> MDYDFKVKLSSERERVEDLFEYEGCKVGRGTYGHVYKAKRKDGKDDKDYALKQIEGTGISMSACREIALLRELKHPNVISLQKVFLSHADRKVWLLFDYAEHDLWHIIKFHRASKANKKPVQLPRGMVKSLLYQILDGIHYLHANWVLHRDLKPANILVMGEGPERGRVKIADMGFARLFNSPLKPLADLDPVVVTFWYRAPELLLGARHYTKAIDIWAIGCIFAELLTSEPIFHCRQEDIKTSNPYHHDQLDRIFNVMGFPADKDWEDIKKMPEHSTLMKDFRRNTYTNCSLIKYMEKHKVKPDSKAFHLLQKLLTMDPIKRITSEQAMQDPYFLEDPLPTSDVFAGCQIPYPKREFLTEEEPDDKGDKKNQQQQQGNNHTNGTGHPGNQDSSHTQGPPLKKVRVVPPTTTSGGLIMTSDYQRSNPHAAYPNPGPSTSQPQSSMGYSATSQQPPQYSHQTHRY;> MAGNFWQSSHYLQWILDKQDLLKERQKDLKFLSEEEYWKLQIFFTNVIQALGEHLKLRQQVIATATVYFKRFYARYSLKSIDPVLMAPTCVFLASKVEEFGVVSNTRLIAAATSVLKTRFSYAFPKEFPYRMNHILECEFYLLELMDCCLIVYHPYRPLLQYVQDMGQEDMLLPLAWRIVNDTYRTDLCLLYPPFMIALACLHVACVVQQKDARQWFAELSVDMEKILEIIRVILKLYEQWKNFDERKEMATILSKMPKPKPPPNSEGEQGPNGSQNSSYSQS;> MAAFGILSYEHRPLKRPRLGPPDVYPQDPKQKEDELTALNVKQGFNNQPAVSGDEHGSAKNVSFNPAKISSNFSSIIAEKLRCNTLPDTGRRKPQVNQKDNFWLVTARSQSAINTWFTDLAGTKPLTQLAKKVPIFSKKEEVFGYLAKYTVPVMRAAWLIKMTCAYYAAISETKVKKRHVDPFMEWTQIITKYLWEQLQKMAEYYRPGPAGSGGCGSTIGPLPHDVEVAIRQWDYTEKLAMFMFQDGMLDRHEFLTWVLECFEKIRPGEDELLKLLLPLLLRYSGEFVQSAYLSRRLAYFCTRRLALQLDGVSSHSSHVISAQSTSTLPTTPAPQPPTSSTPSTPFSDLLMCPQHRPLVFGLSCILQTILLCCPSALVWHYSLTDSRIKTGSPLDHLPIAPSNLPMPEGNSAFTQQVRAKLREIEQQIKERGQAVEVRWSFDKCQEATAGFTIGRVLHTLEVLDSHSFERSDFSNSLDSLCNRIFGLGPSKDGHEISSDDDAVVSLLCEWAVSCKRSGRHRAMVVAKLLEKRQAEIEAERCGESEAADEKGSIASGSLSAPSAPIFQDVLLQFLDTQAPMLTDPRSESERVEFFNLVLLFCELI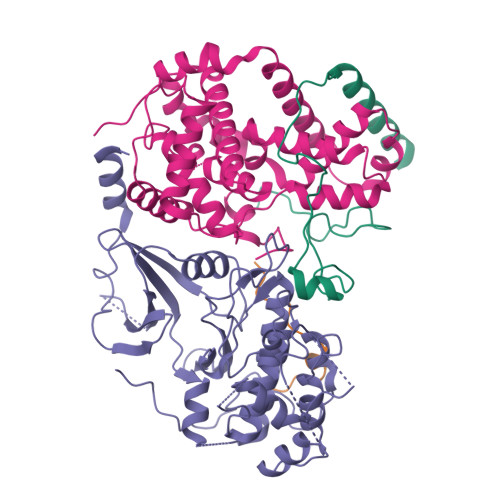RHDVFSHNMYTCTLISRGDLAFGAPGPRPPSPFDDPADDPEHKEAEGSSSSKLEDPGLSESMDIDPSSSVLFEDMEKPDFSLFSPTMPCEGKGSPSPEKPDVEKEVKPPPKEKIEGTLGVLYDQPRHVQYATHFPIPQEESCSHECNQRLVVLFGVGKQRDDARHAIKKITKDILKVLNRKGTAETDQLAPIVPLNPGDLTFLGGEDGQKRRRNRPEAFPTAEDIFAKFQHLSHYDQHQVTAQVSRNVLEQITSFALGMSYHLPLVQHVQFIFDLMEYSLSISGLIDFAIQLLNELSVVEAELLLKSSDLVGSYTTSLCLCIVAVLRHYHACLILNQDQMAQVFEGLCGVVKHGMNRSDGSSAERCILAYLYDLYTSCSHLKNKFGELFSDFCSKVKNTIYCNVEPSESNMRWAPEFMIDTLENPAAHTFTYTGLGKSLSENPANRYSFVCNALMHVCVGHHDPDRVNDIAILCAELTGYCKSLSAEWLGVLKALCCSSNNGTCGFNDLLCNVDVSDLSFHDSLATFVAILIARQCLLLEDLIRCAAIPSLLNAACSEQDSEPGARLTCRILLHLFKTPQLNPCQSDGNKPTVGIRSSCDRHLLAASQNRIVDGAVFAVLKAVFVLGDAELKGSGFTVTGGTEELPEEEGGGGSGGRRQGGRNISVETASLDVYAKYVLRSICQQEWVGERCLKSLCEDSNDLQDPVLSSAQAQRLMQLICYPHRLLDNEDGENPQRQRIKRILQNLDQWTMRQSSLELQLMIKQTPNNEMNSLLENIAKATIEVFQQSAETGSSSGSTASNMPSSSKTKPVLSSLERSGVWLVAPLIAKLPTSVQGHVLKAAGEELEKGQHLGSSSRKERDRQKQKSMSLLSQQPFLSLVLTCLKGQDEQREGLLTSLYSQVHQIVNNWRDDQYLDDCKPKQLMHEALKLRLNLVGGMFDTVQRSTQQTTEWAMLLLEIIISGTVDMQSNNELFTTVLDMLSVLINGTLAADMSSISQGSMEENKRAYMNLAKKLQKELGERQSDSLEKVRQLLPLPKQTRDVITCEPQGSLIDTKGNKIAGFDSIFKKEGLQVSTKQKISPWDLFEGLKPSAPLSWGWFGTVRVDRRVARGEEQQRLLLYHTHLRPRPRAYYLEPLPLPPEDEEPPAPTLLEPEKKAPEPPKTDKPGAAPPSTEERKKKSTKGKKRSQPATKTEDYGMGPGRSGPYGVTVPPDLLHHPNPGSITHLNYRQGSIGLYTQNQPLPAGGPRVDPYRPVRLPMQKLPTRPTYPGVLPTTMTGVMGLEPSSYKTSVYRQQQPAVPQGQRLRQQLQQSQGMLGQSSVHQMTPSSSYGLQTSQGYTPYVSHVGLQQHTGPAGTMVPPSYSSQPYQSTHPSTNPTLVDPTRHLQQRPSGYVHQQAPTYGHGLTSTQRFSHQTLQQTPMISTMTPMSAQGVQAGVRSTAILPEQQQQQQQQQQQQQQQQQQQQQQQQQQYHIRQQQQQQILRQQQQQQQQQQQQQQQQQQQQQQQQQQHQQQQQQQAAPPQPQPQSQPQFQRQGLQQTQQQQQTAALVRQLQQQLSNTQPQPSTNIFGRY;> MSASFVPNGASLEDCHCNLFCLADLTGIKWKKYVWQGPTSAPILFPVTEEDPILSSFSRCLKADVLGVWRRDQRPGRRELWIFWWGEDPSFADLIHHDLSEEEDGVWENGLSYECRTLLFKAVHNLLERCLMNRNFVRIGKWFVKPYEKDEKPINKSEHLSCSFTFFLHGDSNVCTSVEINQHQPVYLLSEEHITLAQQSNSPFQVILCPFGLNGTLTGQAFKMSDSATKKLIGEWKQFYPISCCLKEMSEEKQEDMDWEDDSLAAVEVLVAGVRMIYPACFVLVPQSDIPTPSPVGSTHCSSSCLGVHQVPASTRDPAMSSVTLTPPTSPEEVQTVDPQSVQKWVKFSSVSDGFNSDSTSHHGGKIPRKLANHVVDRVWQECNMNRAQNKRKYSASSGGLCEEATAAKVASWDFVEATQRTNCSCLRHKNLKSRNAGQQGQAPSLGQQQQILPKHKTNEKQEKSEKPQKRPLTPFHHRVSVSDDVGMDADSASQRLVISAPDSQVRFSNIRTNDVAKTPQMHGTEMANSPQPPPLSPHPCDVVDEGVTKTPSTPQSQHFYQMPTPDPLVPSKPMEDRIDSLSQSFPPQYQEAVEPTVYVGTAVNLEEDEANIAWKYYKFPKKKDVEFLPPQLPSDKFKDDPVGPFGQESVTSVTELMVQCKKPLKVSDELVQQYQIKNQCLSAIASDAEQEPKIDPYAFVEGDEEFLFPDKKDRQNSEREAGKKHKVEDGTSSVTVLSHEEDAMSLFSPSIKQDAPRPTSHARPPSTSLIYDSDLAVSYTDLDNLFNSDEDELTPGSKKSANGSDDKASCKESKTGNLDPLSCISTADLHKMYPTPPSLEQHIMGFSPMNMNNKEYGSMDTTPGGTVLEGNSSSIGAQFKIEVDEGFCSPKPSEIKDFSYVYKPENCQILVGCSMFAPLKTLPSQYLPPIKLPEECIYRQSWTVGKLELLSSGPSMPFIKEGDGSNMDQEYGTAYTPQTHTSFGMPPSSAPPSNSGAGILPSPSTPRFPTPRTPRTPRTPRGAGGPASAQGSVKYENSDLYSPASTPSTCRPLNSVEPATVPSIPEAHSLYVNLILSESVMNLFKDCNFDSCCICVCNMNIKGADVGVYIPDPTQEAQYRCTCGFSAVMNRKFGNNSGLFLEDELDIIGRNTDCGKEAEKRFEALRATSAEHVNGGLKESEKLSDDLILLLQDQCTNLFSPFGAADQDPFPKSGVISNWVRVEERDCCNDCYLALEHGRQFMDNMSGGKVDEALVKSSCLHPWSKRNDVSMQCSQDILRMLLSLQPVLQDAIQKKRTVRPWGVQGPLTWQQFHKMAGRGSYGTDESPEPLPIPTFLLGYDYDYLVLSPFALPYWERLMLEPYGSQRDIAYVVLCPENEALLNGAKSFFRDLTAIYESCRLGQHRPVSRLLTDGIMRVGSTASKKLSEKLVAEWFSQAADGNNEAFSKLKLYAQVCRYDLGPYLASLPLDSSLLSQPNLVAPTSQSLITPPQMTNTGNANTPSATLASAASSTMTVTSGVAISTSVATANSTLTTASTSSSSSSNLNSGVSSNKLPSFPPFGSMNSNAAGSMSTQANTVQSGQLGGQQTSALQTAGISGESSSLPTQPHPDVSESTMDRDKVGIPTDGDSHAVTYPPAIVVYIIDPFTYENTDESTNSSSVWTLGLLRCFLEMVQTLPPHIKSTVSVQIIPCQYLLQPVKHEDREIYPQHLKSLAFSAFTQCRRPLPTSTNVKTLTGFGPGLAMETALRSPDRPECIRLYAPPFILAPVKDKQTELGETFGEAGQKYNVLFVGYCLSHDQRWILASCTDLYGELLETCIINIDVPNRARRKKSSARKFGLQKLWEWCLGLVQMSSLPWRVVIGRLGRIGHGELKDWSCLLSRRNLQSLSKRLKDMCRMCGISAADSPSILSACLVAMEPQGSFVIMPDSVSTGSVFGRSTTLNMQTSQLNTPQDTSCTHILVFPTSASVQVASATYTTENLDLAFNPNNDGADGMGIFDLLDTGDDLDPDIINILPASPTGSPVHSPGSHYPHGGDAGKGQSTDRLLSTEPHEEVPNILQQPLALGYFVSTAKAGPLPDWFWSACPQAQYQCPLFLKASLHLHVPSVQSDELLHSKHSHPLDSNQTSDVLRFVLEQYNALSWLTCDPATQDRRSCLPIHFVVLNQLYNFIMNML> MFIKQSEKNTPKCLYKKKGKVRVLLTGSCKKLNTWKMHLWPVSPPQLLRIPPRNAELGEGTKIDDCNILQSMTLPQANVLIMLTPTRVLIYNFKPMALVASHERTMASLKEFGDNRSMKRSAPYNDIIEGLISKKDSQYLLWHQGKLIFYVMTDKNFLLTYQILKNCTNEIIFKEYGIPVIEPLLMSEEEANSAEYDYNNDDDTLTVFDKNSSSRIIQNGFGITKEKGFLHFLSNQENIDELPVKKLELRLKVVLKFDYEIIDMIGIKTFSKVGDGRYEEVLIVLFPHGLQILTISDFKVSKSSLVEVKKGSKTIVCNKQLMVLSHDSVEKQTIVSIIDIEKQAVEAIPLTDTPDELLTCLEVNGYLVVVYKEKIICFDTRIKKVSHSWKPPFVIKLCDKINDKILLLVSEDSVNIHFYTEFGNLLFATYFDEDDYNGDNNNDNSKDKNEKKAAEYKISDFVCLDKSLITVSHSGKYQVWKLWEEIKQTQFDFRNPKCYVLTNTNNDVIIYSPVTSSSINNDNLQVIKLPTKTFNNHIAFVKINSSLRLFATYVSNKNILLIHNLETNMWSSFADQNVLDLHWLGDNYLVCHMKNDDGSTNLKCLQIPLQEANPDVELSDYVMWEYNVPENTIVFSLHVNTLSRYKLLKMKSKNHNASEKQPDALLKTAEIILVTDTQTIVFDVISTVHPCGLNIIKKFYQYLKINIPIDVLPNKIEWIINMKEGLLFFADRKFIKLGKVDGGGWQTLTLLDNIEKIIDVIRDEIFVVQGHNYVVYSLEDLWDDKKPLVSIPIEEDLYPISTTPETATTHTLHCIFNARFSKLVVKHQIYLDQLILAKLEDNTDLEDISHNYRFLKPYKFALEKILSTKILRSDSLDDILKLIKMYDNTDPEHNISPPTHSGMLEIISNCLRKIETKYWNHLFTNLKMTPRDLLALCIEENEAKMLGVLLLVFLNYDEKDLGDDLHFKKSDLGTEESKALNDNSTKKSEKSVTNLLKXXXXXXXXXXXXXXXXXXATDXXXXXXXXXXXXXXXXXXXXXDRENNTQXXXXXXXXXX;> MRAHRIDTFLIRENIKLEIIHESNSYFGGEHISIAFRFKHLGSQHELF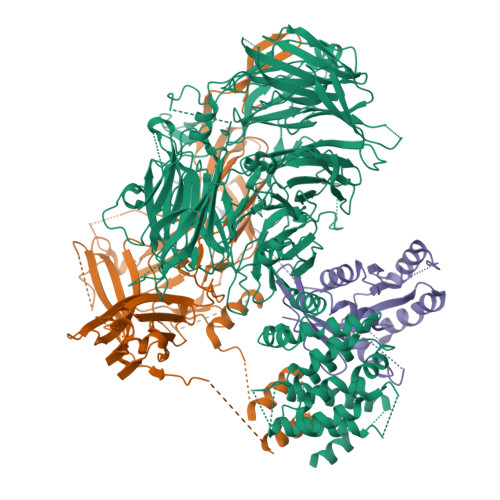NYKEKLLTVDKAVEEKLEQQAKVQDDGEGTMENQTWSLKSLLGAFKRTGEPEESVDVDNMKMLNESKMLREKIQKQMYFHQPVTLISGYVQISGVFQYDSEVISESKFKQDEVKMVGLDIVPGHTTNSVLALEDGEHFKGKRNLTNYLNSDYTNVTNGLLFSESGSRGRTGTYNERTLMISNDTSIKTLPLLLIPQTLLFSEISLEPGEVRTFYFKSTKLPKDICPSYSSSKVASINYTLEVGADVLSDDNIEKFSNRVPITIAPYISSNAEQYTSRLDKPAIILKTGNIKELKPRLFTRKVSTASAVSFGRRKSSIIDIDSPLEDNEFVXXXXXXXXXXXXSNQNVSRXXXXXXXXXXXXQFGKDEDSSDPEPNDSHFSNEMVTSAESSLRSDAVTKRRKSYSVRDNISNLEQKMWNDCSLVKSDENSNLLPQLINLQNAYQINRNNETMAKVSLSAPFYKTTDDINLVIELDPITTPLLKVTSLTVSLESFEIINPKYKTEGKGIGSKPKGNSVYEKHFICFDECKSVSVKLLPPRSPTNQITGQFKTDVFQHKWMIGLKFVIIAKTESITLDQFYEDKKGILFHSKENLEGEEFTCYVPIPILCTSEDFMGW;> MSRSGKSLTKYKIVFLGEQGVGKTSLITRFMYDTFDDHYQATIGIDFLSKTMYLDDKTIRLQLWDTAGQERFRSLIPSYIRDSRVAIIVYDITKRKSFEYIDKWIEDVKNERGDENVILCIVGNKSDLSDERQISTEEGEKKAKLLGAKIFMETSTKAGYNVKALFKKIAKSLPEFQNSESTPLDSENANSANQNKPGVIDISTAEEQEQSACQC>APAADAAQAHDPLSVQTGSDIPASVHMPTDQQRDYIKREVMVPMRDGVKLYTVIVIPKNARNAPILLTRTPYNAKGRANRVPNALTMREVLPQGDDVFVEGGYIRVFQDIRGKYGSQGDYVMTRPPHGPLNPTKTDETTDAWDTVDWLVHNVPESNGRVGMTGSSYEGFTVVMALLDPHPALKVAAPESPMVDGWMGDDWFHYGAFRQGAFDYFVSQMTARGGGNDIPRRDADDYTNFLKAGSAGSFATQAGLDQY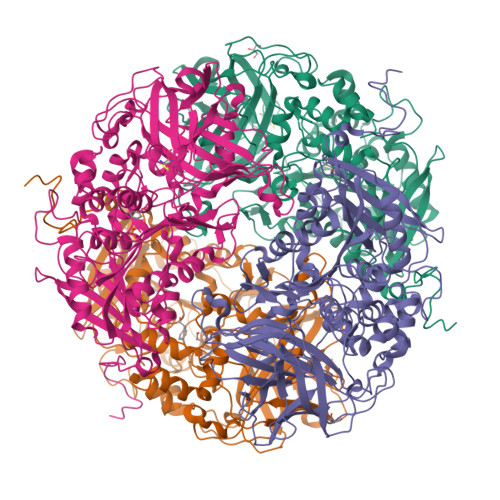PFWQRMHAHPAYDAFWQGQALDKILAQRKPTVPMLWEQGLWDQEDMWGAIHAWQALKDADVKAPNTLVMGPWRHSGVNYNGSTLGPLEFEGDTAHQYRRDVFRPFFDEYLKPGSASVHLPDAIIYNTGDQKWDYYRSWPSVCESNCTGGLTPLYLADGHGLSFTHPAADGADSYVSDPAHPVPFISRPFAFAQSSRWKPWLVQDQREAESRPDVVTYETEVLDEPVRVSGVPVADLFAATSGTDSDWVVKLIDVQPAMTPDDPKMGGYELPVSMDIFRGRYRKDFAKPEALQPDATLHYHFTLPAVNHVFAKGHRIMVQIQSSWFPLYDRNPQKFVPNIFDAKPADYTVATQSIHHGGKEATSILLPVVKQKLGPEQKLISEEDLNSAVDHHHHHH[4x]> GSMGSLTKNDNLHIFLVCFIGQGVVNPMLRLGKAFASKGLLVTLSAPEIVGREIRKANNLNDDQSIKVGNGMIRFEFFDDGWESVNGSKPFDVGVYINHLDQAGRQKLPIMLKKHEESGTPVSCLILNPLVPWVADVADSLQIPCATLWVQSCASFSAYYHYHHGLVPFPTESEPEIDVQLPGMPLLKYDEVPDYLHPRTPYPFFGTNILGQFKNLSKNFCILMDTFYELEHETIDSITKICPIKPIGPLFKIPKDPSSNGITGNFMKVDDCKEWLDTRPPSTVVYVSVGSVVYLKQEQVTEMAYGILNSEVSFLWVLRPPSKRIGTEPHVLPEEFWEKAGDRGKVVQWSPQEQVLAHPATAAFLTHCGWNSTQEAISSGVPVITFPQFGDQVTNAK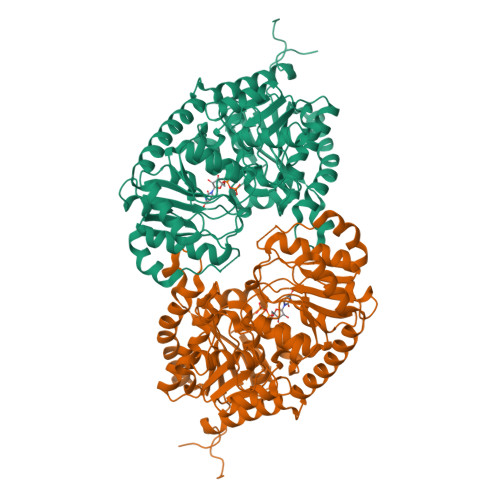FLVEEFKVGVRLSRGELENRIITRDEVERALREITSGPKAEEVKENALKWKKAAEETVAKGGNSERNLVEFIEEVARKTGSKHESHVG>[2x]MSGTRASNDRPPGTGGVKRGRLQQEAAATGSRVTVVLGAQWGDEGKGKVVDLLATDADIVSRCQGGNNAGHTVVVDGKEYDFHL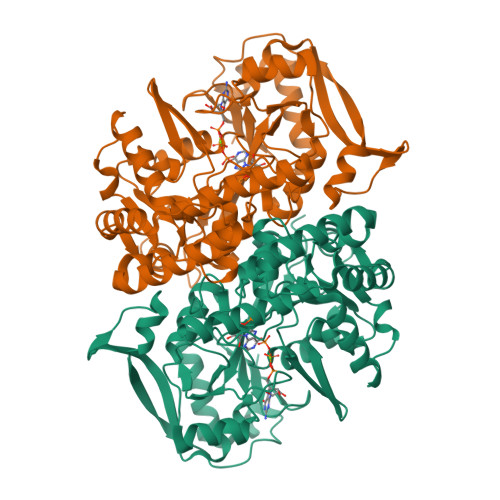LPSGIINTKAVSFIGNGVVIHLPGLFEEAEKNEKKGLKDWEKRLIISDRAHLVFDFHQAVDGLQEVQRQAQEGKNIGTTKKGIGPTYSSKAARTGLRICDLLSDFDEFSARFKNLAHQHQSMFPTLEIDVEGQLKRLKGFAERIRPMVRDGVYFMYEALHGPPKKVLVEGANAALLDIDFGTYPFVTSSNCTVGGVCTGLGIPPQNIGDVYGVVKAYTTRVGIGAFPTEQINEIGDLLQNRGHEWGVTTGRKRRCGWLDLMILRYAHMVNGFTALALTKLDILDVLSEIKVGISYKLNGKRIPYFPANQEILQKVEVEYETLPGWKADTTGARKWEDLPPQAQSYVRFVENHMGVAVKWVGVGKSRESMIQLF>AQVINTFDGVADYLQTYHKLPDNYITKSEAQALGWVASKGNLADVAPGKSIGGDIFSNREGKLPGK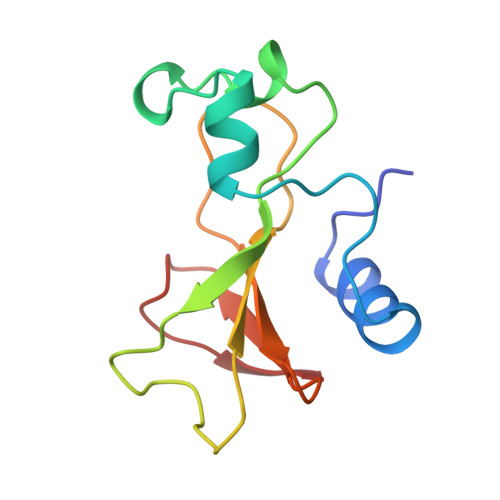SGRTWREADINYTSGFRNSDRILYSSDWLIYKTTDHYQTFTKIR[3x]>[8x]MEIKRRTQEERSAATREALITGARKLWGLRGY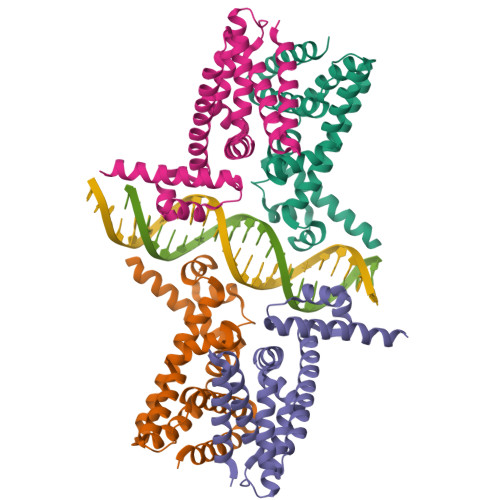AEVGTPEIATEAGVTRGAMYHQFADKAALFRDVVEVVEQDVMARMATLVAASGAATPADAIRAAVDAWLEVSGDPEVRQLILLDAPVVLGWAGFRDVAQRYSLGMTEQLITEAIRAGQLARQPVRPLAQVLIGALDEAAMFIATADDPKRARRETRQVLRRLIDGMLNGKLAAALEHHHHHH>[2x]GSCSSKPANTAKGEKGSDKTGKDLELKLSFQEGIAPGESLNEKLDFMEKLGVVGFEPGGGGLAGRVNEIKQALNGRNIKVSAICAGFKGFILSTDPAIRKECMDTMKEIIAAAGEL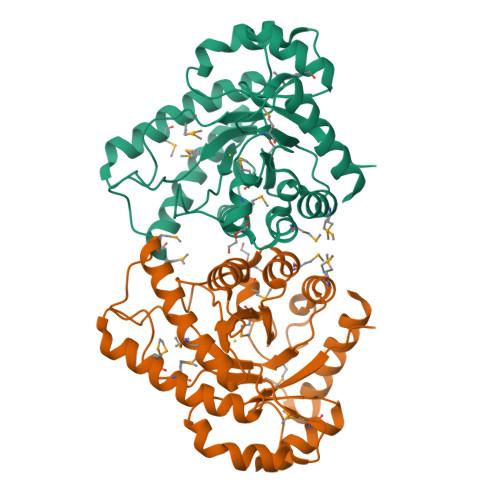GSTGVIIVPAFNGQVPALPHTMETRDFLCEQFNEMGTFAAQHGTSVIFEPLNRKECFYLRQVADAASLCRDINNPGVRCMGDFWHMTWEETSDMGAFISGGEYLQHVHVASRKRRSMPGEDGDADNYINGFKGLKMIGYNNYVSFECGCQGDRNVVVPAAVKLLREQWEQA>[2x]TFGTFQDAYLSQLRDIYHSPEFRNAPRGQASRERIGAGFRLLDPVQRHISVPARRANVVFNFAEALWYLSGSDRLDFIQYYAPGIAAYSADGRTLRGTAYGPRIFRHPAGGVNQWENVVKTLTDDPDSKRAVIQIFDPRELAVADNIDVACTLALQFLIRDGLLCGIGYMRANDAFRGAVSDVFSFTFLQEFTARYLGLGIGTYHHVVGSVHIYDSDARWAERVLDAATPDGGPRPGFPAMPDGDNWPHVRRVLEWEERLRTNAARLSADALDALDLPAYWKHVVALFEAHRQVRHEDTPDRALLAALPEVYRQSLAVKWPGHFG

We previously demonstrated that MilA, a CMP hydroxymethylase in the mildiomycin biosynthetic gene cluster in Streptomyces rimofaciens ZJU5119, can convert CMP to hmCMP12. MilA and CH are akin to the superfamily of thymidylate synthases (TS), which transfers a methyl group from CH2THF to dUMP to form dTMP in the de novo thymidylate synthesis pathway and, hence, DNA synthesis. In this study, we demonstrated that MilA has a substrate preference for CMP (kcat/KM = 39.2 mM−1 min−1) over dCMP (kcat/KM = 7.84 mM−1 min−1), and thus offers an opportunity to investigate the mechanism by which conserved TS evolves the preference for ribosyl over 2′-deoxyribosyl groups. In the structures of apo MilA and its complexes with various substrates, MilA are all homodimers.

Subsequently, the structures of MilA‒CMP, MilA‒dCMP and MilA‒hmCMP complexes were refined to 1.65 Å, 2.10 Å and 1.80 Å resolution, respectively. Through a comparison of the active site structures of the TS-dUMP, CH‒dCMP, MilA-dCMP and MilA‒CMP complexes, it was found that the 3′-hydroxyl groups of the sugar moiety of substrates adopt two different conformations when complexed with MilA or TS/CH; the 3′-carbon together with its 3′-OH of deoxyribose motif has a dramatic torsion (with 3′-C set as the vertex, the angle from 6′-O to 3′-O is increased from 102.3°/105.3° to 136.4°) in MilA-dCMP relative to TS-dUMP/CH-dCMP. However, in MilA-dCMP, the 3′-hydroxyl group of dCMP forms one hydrogen bond with the Lys-133′ and another intramolecular hydrogen bond with the phosphate group. The main reason for this difference is that Ala176 in MilA is replaced by a serine, Ser167/Ser169, in TS/CH. In contrast, Ala176, with its much smaller side-chain methyl group, is the corresponding residue for TS-Ser167/CH-Ser169 in MilA and makes the larger room. Therefore, both CMP and dCMP are able to fit into the substrate-binding pocket of MilA. Hence, MilA can not only can utilize CMP, but also can use dCMP as its substrate like CH and TS. The KM for CMP was 0.0719 mM, 3.4-fold lower than that for dCMP (KM = 0.245 mM), demonstrating that CMP was a better substrate than dCMP for MilA. By contrast, its counterpart residue in MilA is lysine 133′, which formed hydrogen bonds with 3′-hydroxyl group of dCMP or CMP in respective protein/substrate complex (panel 2&3).>SMQLNQYKLQSEIGKGAYGVVRLAYNESEDRHYAMKVLSKKKLLKQYGFPRRPPPRGSQAAQGGPAKQLLPLERVYQEIAILKKLDHVNVVKLIEVLDDPAEDNLYLVFDLLR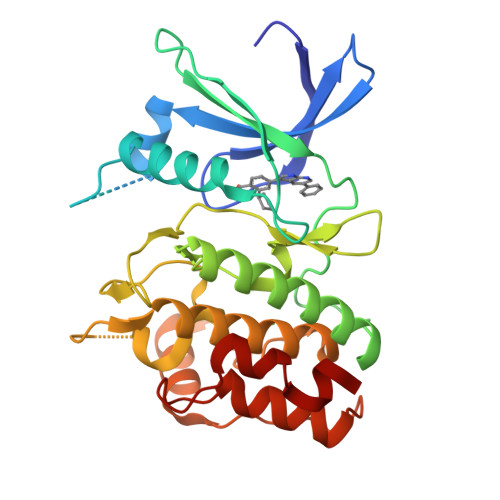KGPVMEVPCDKPFSEEQARLYLRDVILGLEYLHCQKIVHRDIKPSNLLLGDDGHVKIADFGVSNQFEGNDAQLSSTAGTPAFMAPEAISDSGQSFSGKALDVWATGVTLYCFVYGKCPFIDDFILALHRKIKNEPVVFPEEPEISEELKDLILKMLDKNPETRIGVPDIKLHPWVTK[4x]>[5x]MDSGDGQDLRAFVHDSPEETETTQRLTKLLTNSPIPTEELVNNLPLFLRRHQMTDLLSMDALYRQVLDVPGVIMEFGVRFGRHLGTF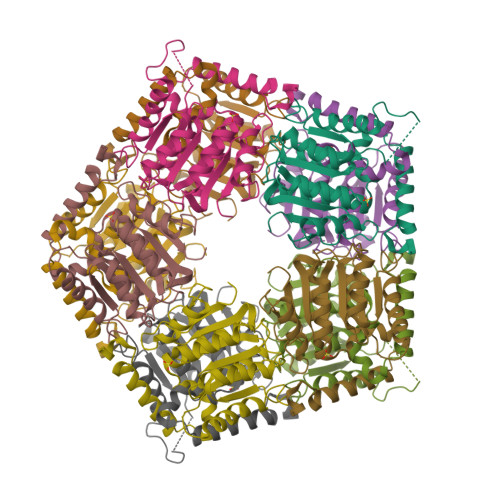AALRGVYEPYNPLRRIVGFDTFTGFPDVNDVDRVGPTAYQGRFAVPGGYPAYLKEVLDAHECSDFFGHVTQRSVLVEGDVRETVPRYLAENPQTVIALAYFDLDLYEPTKAVLEAIRPYLTKGSIVAFDELDNPKWPGENIAMRKVLGLDHAPLRLLPGRPAPAYLRWGD>GQNHHEVVKFMDVYQRSYCHPIETLVDIFQEYPDEIEYIFKPSCVPLMRCGGCCNDEGLECVPTEESNITMQIMRIKPHQGQHIGEMSFLQHNKCECRPKKD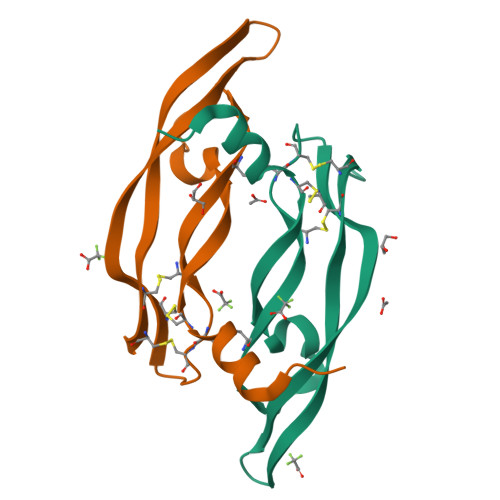[6x]> WYGYWK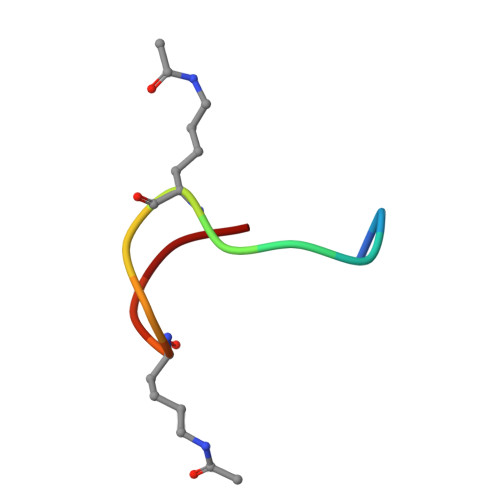VPKRKC> GPLGSMSLRPCFVSLIDESDKPILIYV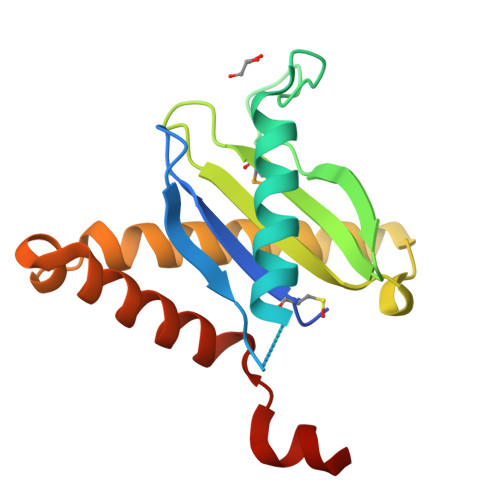PNEAENEMNDVLKYNVLSNISLDYFESALVEWHSLDSKPLLKSIFQLEGVSVFAMLIKQTGLKIVIGFEQKSLSGADDEFEAINQIFETVRKIYIRVKCNPLLVSGDEKSIIKSLERKFDELFISTEVELLAAAS>TNYYYSAVERNNLMRLSQSIPFVPVPPRGEPVTVYRLEESSPSILNNSMSSWSQLGLCAKIEFLSKEEMGGGLRRAVKVLCTWSEHDILKSGHLYII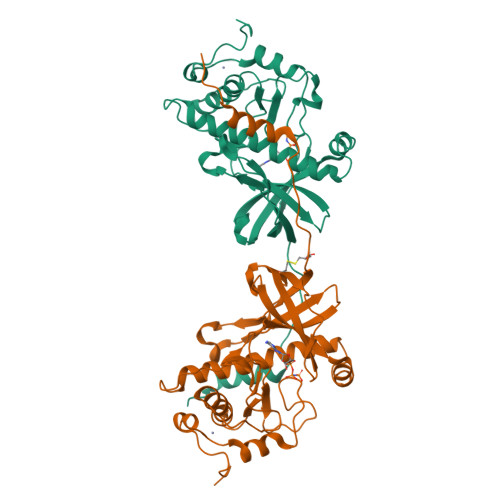KSFLPEVINTWSSIYKEDTVLHLCLREIQQQRAAQKLTFAFNQMKPKSIPYSPRFLEVFLLYCHSAGQWFAVEECMTGEFRKYNNNNGDEIIPTNTLEEIMLAFSHWTYEYTRGELLVLDLQGVGENLTDPSVIKAEEKRSCDMVFGPANLGEDAIKNFRAKHHCNSCCRKLKLPDLKRNDYT[2x]> MASMTGGQQMGRGSIVAASTIPGSAATLNTSITKNIQNGNAYIDLYDVKLGKIDPLQLIVLEQGF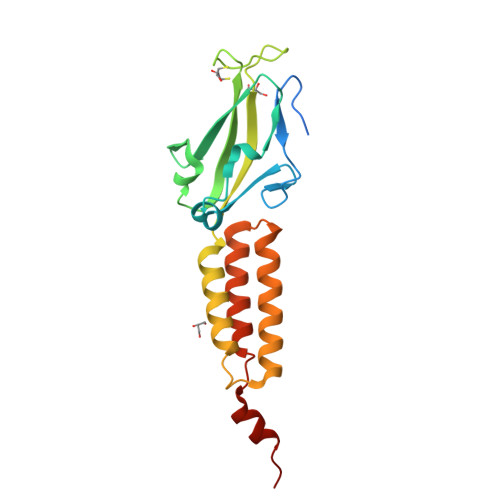TAKYVFRQGTKYYGDVSQLQSTGRASLTYNIFGEDGLPHVKTDGQIDIVSVALTIYDSTTLRDKIEEVRTNANDPKWTEESRTEVLTGLDTIKTDIDNNPKTQTDIDSKIVEVNELEKLLVLKLAAALEHHHHHH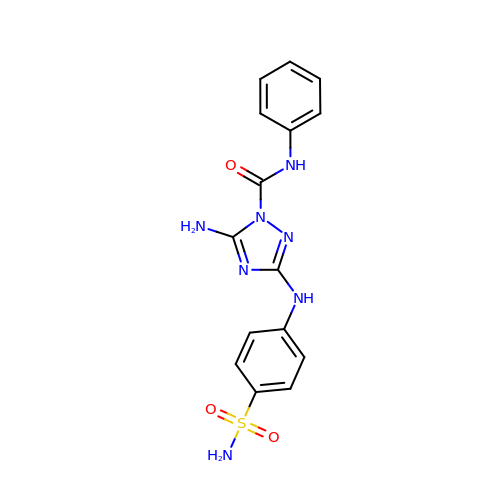5-amino-N-phenyl-3-[(4-sulfamoylphenyl)amino]-1H-1,2,4-triazole-1-carboxamide | C15 H15 N7 O3 S | ZQFUBCAVNORBSG-UHFFFAOYSA-N> DEFEMIKRNTSEIISEEELREVLKKDEKSAGIGFEPSGKIHLGHYLQIKKMIDLQNAGFDIIILLADLHAYLNQKGELDEIRKIGDYNKKVFEAMGLKAKYVYGSPFQLDKDYTLNVYRLALKTTLKRARRSMELIAREDENPKVAEVIYPIMQVNTSHRLGVDVAVGGMEQRKIHMLARE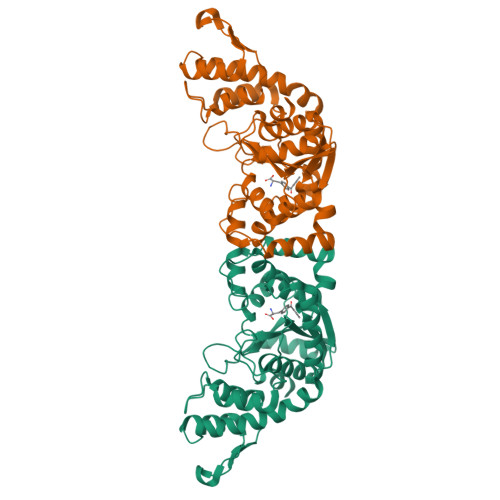LLPKKVVMIHNPVLTGLDGEGKMSSSKGNFIAVDDSPEEIRAKIKKAYCPAGVVEGNPIMEIAKYFLEYPLTIKRPEKFGGDLTVNSYEELESLFKNKELHPMDLKNAVAEELIKILEPIRKRLL> MNLMTTITGVVLAGGKARRMGGVDKGLLELNGKPLWQHVADALMTQLSHVVVNANRHQEIYQASGLKV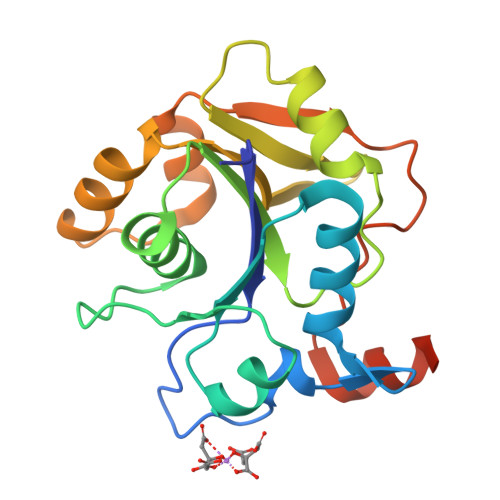IEDSLADYPGPLAGMLSVMQQEAGEWFLFCPCNTPYIPPDLAARLNHQRKDAPVVWVHDGERDHPTIALVNRAIEPLLLEYLQAGERRVMVFMRLAGGHAVDFSDHKDAFVNVNTPEELARWQEKRSHHHHHH>[2x]MTGQAAGPAAGPAAGQATKHAGGRRPGETRTREAILTAARVCFAERGFDATSLRRIAETAGVDQSLVHHFYGTKENLFLQALELPGKIEEAITAAAQGGLDGIGERVVRAHLSVWDDVSSR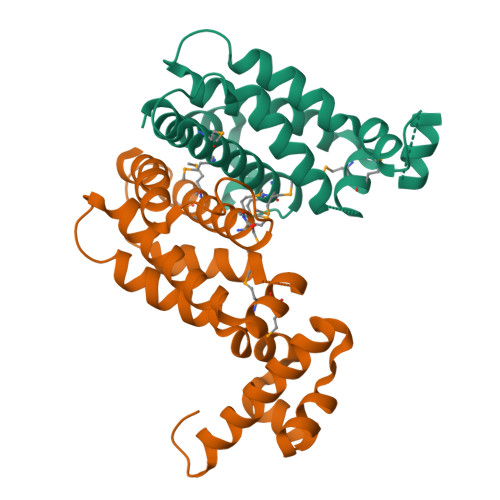PALMTMVRSAAIHRAAAARLRETATGILARALGGVITGEDAMLRTSMVATQLVGLAMMRYVAHLEPLASADTDTVARHYGRAVQAIVTDRD>GGGTTGGGTTGGGTT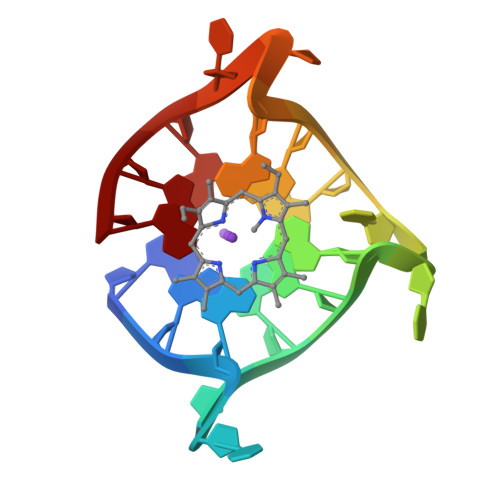GGG[2x]>MSVIKQVMKTKLHLEGTVNGHDFTIEGKGEGKPYEGLQHMKMTVTKGAPLPFSVHILTPSHMYGSKPFNKYPADIPDYHKQSFPEGMSWERSMIFEDGGVCTASNHSSINLQENCFIYDVKFHGVNLPPDGPVMQKTIAGWEPSVETLYVRDGMLKSDTAMVFKLKGGGHHRVDFKTTYKAKKPVKLPEFHFVEHRLELTKHDKDFTTWDQQEAAEGHFSPLPKALP[4x]

Anthozoan chromoproteins are highly pigmented, diversely coloured and readily produced in recombinant expression systems. Here, high-resolution X-ray crystal structures of four open-source chromoproteins, gfasPurple, amilCP, spisPink and eforRed, are presented. Like GFP, chromoprotein monomers have a β-barrel structure that contains a chromophore, which is autocatalytically constructed from adjacent X–tyrosine–glycine residues encoded within the protein sequence itself.

The chromophores are trans and noncoplanar in gfasPurple, amilCP and spisPink, while that in eforRed is cis and noncoplanar, and also emits fluorescence. The reddish appearance of eforRed can be attributed to its intense, red-shifted fluorescence emission that peaks at 602 nm. Studies of photo-switchable fluorescent proteins indicate that coplanarity is more essential for fluorescence than a cis chromophore conformation, as fluorescence is also observed in mutants containing trans but coplanar chromophore variants. The other requirement in fluorescent chromoprotein variants is thought to be a histidine (His197) π-stacking with the tyrosyl moiety, which is observed in eforRed but not dsRed. Most notably, an unusual hydroxyl-to-methionine hydrogen bond was observed in eforRed between the tyrosyl moiety and Met161, while the equivalent Met159 in gfasPurple and amilCP only forms van der Waals interactions.>[4x]KDKKKGKKNIPMTEIQTTGTQDRAIWVKLLWKISYPVIHNLAEGTLHQNMPIETRSGETAGYKDMTHLEAVGRTLAGVAPWLALPDDDTEEGKLRKQMREEVLKGLKNAVDPASPDLLNFTKHAQPIVDAAYLVHAFLRAPKALWEPLDEVTKERYIKSFQSLRDRTGAYNNWLLFTGLTESFLLGKGVQYDQFRIRVSKNKVKEWYVGDGWYSDGPSFSMDNYNAYVMHSMMVAMLENLLPKRWASQKELDEAMNRMIRHSEFCERMIAPDGTYPAFGRSVTYRTAAFQSLADVALRKKLPSHVSPAQVRCALTAVHRNMYEGNQNFDKDGWLVLGFNGHQPECADGYTSTGSLYMATLSFLPLGLPADDPFWTDAYADWTSKKAWKGGHLHKDYKVEY

Here we show that components of a (PUL) from Bacteroides caccae have activities consistent with comprising a unique pathway for depolymerization of chondroitin sulfate, a common GAG. After prior desulfation by an endo-sulfatase, BcSulf, to produce unsulfated chondroitin from chondroitin sulfate, the depolymerization pathway begins with the activity of a polysaccharide lyase from family 35, BcPL35. BcPL35 activity is coupled with BcGH88, an exo-β-uronyl hydrolase, and presumably BcGH109, a confirmed α/β-N-acetylgalactosaminidase. The most unique feature of the pathway is a β-D-glucuronate dehydratase, BcGDH, which we show through structural and functional analyses primes saturated non-reducing end β-D-glucuronate residues for hydrolysis by BcGH88.

BcGDH is a member of a large family previously classified as glycoside hydrolase family 154. Instead, the evidence using chondrosine as a mimic of the natural substrate clearly supports that this enzyme, which we refer to as BcGDH, is a β-D-glucuronic acid dehydratase that converts the terminal β-1,4-linked GlcA into a terminal Δ4,5-unsaturated uronic acid and, therefore, renders the sugar a substrate for BcGH88. We solved the X-ray crystal structure of BcGDH and refined it in the spacegroup P21 to 2.25 Å resolution. The resulting structure comprised a well-organized tetramer in the asymmetric unit that is predicted by PISA analysis to be stable in solution. The structure shows a pronounced slot on the surface of each monomer that is slightly tilted toward the center of the tetramer (circled region). An analysis of the surface residues of BcGDH for conservation in the family revealed the residues in the slot to be highly conserved and likely to comprise the active site. Residues on the surfaces making up the quaternary structure interfaces were not conserved, possibly indicating different, or lacking, quaternary structures among other family members. Based on this analysis, we chose to make alanine mutations of 10 residues in the putative active site (E74 A, R78 A, N176 A, N177 A, W178 A, F181 A, Y229 A, R285 A, Y289 A, and Y354 A) and assay them for activity. None of the mutants had activity when using up to 10 mM chondrosine, despite displaying thermal stability similar to the unmutated enzyme. None of the structures display an active site architecture consistent with typical glycoside hydrolase activity (i.e., potential acid/base or nucleophilic side chains in appropriate proximity to the substrate glycosidic bond).> MPFTIDSARGIFPNTLAADVVPATIARFSQLNAEDQLALIWFAYLEMGKTLTIAAPGAASMQLAENALKEIQAMGPLQQTQAMCDLANRADTPLCRTYASWSPNIKLGFWYR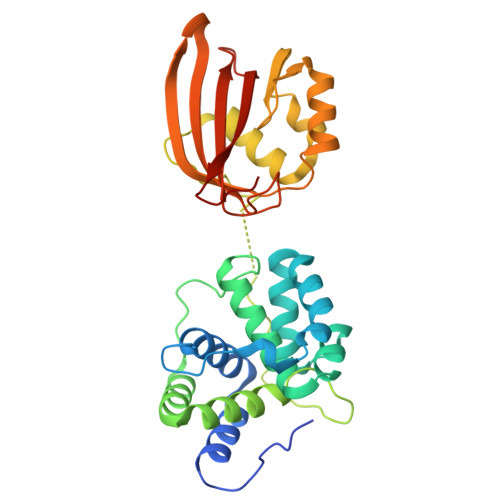LGELMEQGFVAPIPAGYQLSANANAVLATIQGLESGQQITVLRNAVVDMGFTAGKDGKRIAEPVVPPQDTASRTKVSIEGVTNATVLNYMDNLNANDFDTLIELFTSDGALQPPFQRPIVGKENVLRFFREECQNLKLIPERGVTEPAEDGFTQIKVTGKVQTPWFGGNVGMNIAWRFLLNPEGKIFFVAIDLLASPKELLNFAR>MGESERSEAFGIPRDSPLSSGDAAELEQLRREAAVLREQLENAVGSHAPTRSARDIHQLEARIDSLAARNSKLMETLKEARQQLLALREEVDRLGQPPSGYGVLLATHDDDTVDVFTSGRKMRLTCSPNIDAASLKKGQTVRLNEALTVVEAGTFEAVGEISTLREILADGHRALVVGHADEERVVWLADPLIAEDLPDGLPEALNDDTRPRKLRPGDSLLVDTKAGYAFERIPKAEVEDLVLEEVPDVSYADIGGLSRQIEQIRDAVELPFLHKELYREYSLRPPKGVLLYGPPGCGKTLIAKAVANSLAKKMAEVRGDDAHEAKSYFLNIKGPELLNKFVGETERHIRLIFQRAREKASEGTPVIVFFDEMDSIFRTRGTGVSSDVETTVVPQLLSEIDGVEGLENVIVIGASNREDMIDPAILRPGRLDVKIKIERPDAEAAQDIYSKYLTEFLPVHADDLAEFDGDRSACIKAMIEKVVDRMYAEIDDNRFLEVTYANGDKEVMYFKDFNSGAMIQNVVDRAKKNAIKSVLETGQPGLRIQHLLDSIVDEFAENEDLPNTTNPDDWARISGKKGERIVYIRTLVTGKSSSASRAIDTESNLGQYL[6x];> GSMAQEQTKRGGGGGDDDDIAGSTAAGQERREKLTEETDDLLDEIDDVLEENAEDFVRAY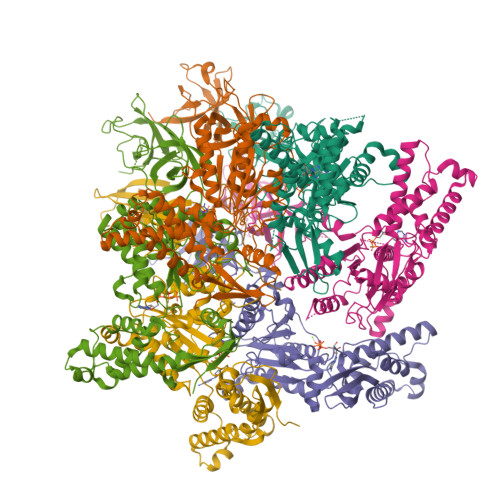VQKGGQ4-(dimethylamino)-N-[(5Z)-9-[[4-[5-(4-fluorophenyl)-3-methyl-2-methylsulfanyl-imidazol-4-yl]pyridin-2-yl]amino]-11,12-dihydrobenzo[c][1,2]benzodiazocin-2-yl]butanamide 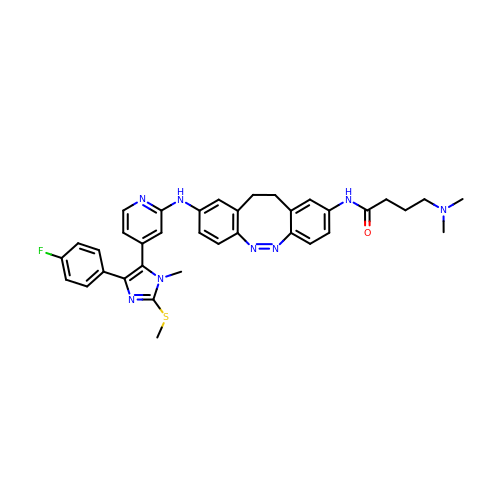| C36 H37 F N8 O S | RSENMMKQMACIQF-RPYQSRGHSA-N> GAMDPDELPLDEHCERLPYDASKWEFPRDRLKLGKPLGRGAFGQVIEADAFGIDKTATCRTVAVKMLKEGATHSEHRALMSELKILIHIGHHLNVVNLLGACTKPGGPLMVI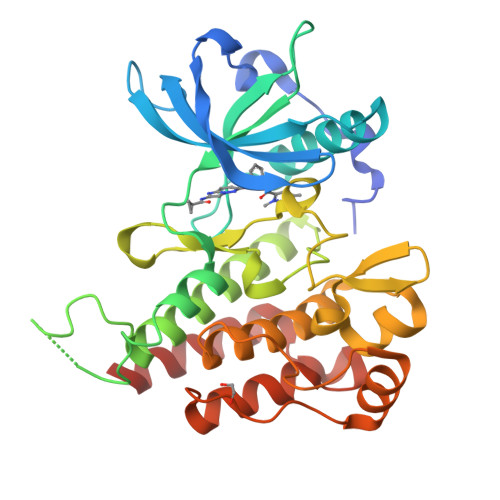VEFCKFGNLSTYLRSKRNEFVPYKEAPEDLYKDFLTLEHLICYSFQVAKGMEFLASRKCIHRDLAARNILLSEKNVVKICDFGLARDIYKDPDYVRKGDARLPLKWMAPETIFDRVYTIQSDVWSFGVLLWEIFSLGASPYPGVKIDEEFCRRLKEGTRMRAPDYTTPEMYQTMLDCWHGEPSQRPTFSELVEHLGNLLQANAQQD>[2x]MQYHRIPHSSLEVSTLGLGTMTFGEQNSEADAHAQLDYAVAQGINLIDVAEMYPVPPRPETQGLTETYVGNWLAKHGSREKLIIASKVSGPSRNNDKGIRPDQALDRKNIREALHDSLKRLQTDYLDLYQVHWPQRPTNC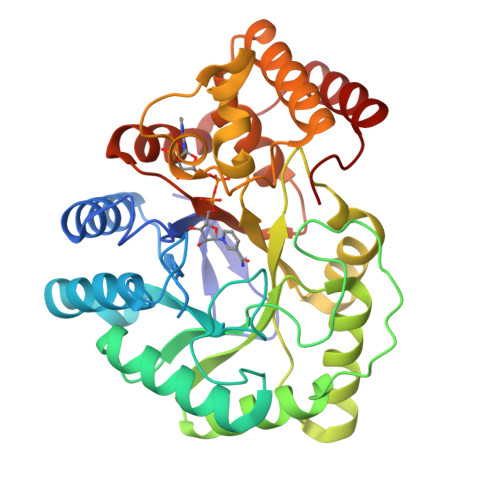FGKLGYSWTDSAPAVSLLDTLDALAEYQRAGKIRYIGVSNETAFGVMRYLHLADKHDLPRIVTIQNPYSLLNRSFEVGLAEVSQYEGVELLAYSCLGFGTLTGKYLNGAKPAGARNTLFSRFTRYSGEQTQKAVAAYVDIARRHGLDPAQMALAFVRRQPFVASTLLGATTMDQLKTNIESLHLELSEDVLAEIEAVHQVYTYPAP> GSDGDALLKPCKLGDMQCLSSATEQFLEKTSKG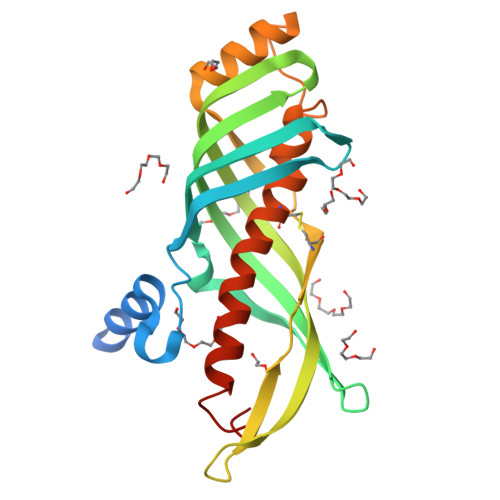IPQYDIWPIDPLVVTSLDVIAPSDAGIVIRFKNLNITGLKNQQISDFQMDTKAKTVLLKTKADLHIVGDIVIELTEQSKSFTGLYTADTNVIGAVRYGYNLKNDDNGVQHFEVQPETFTCESIGEPKITLSSDLSSALEKDSGNNSLEPDMEPLKTLRQAAICKIAEACYISVVHNIRASAKILPASSFFENLN>[3x]GGARSDKLLYQAKLA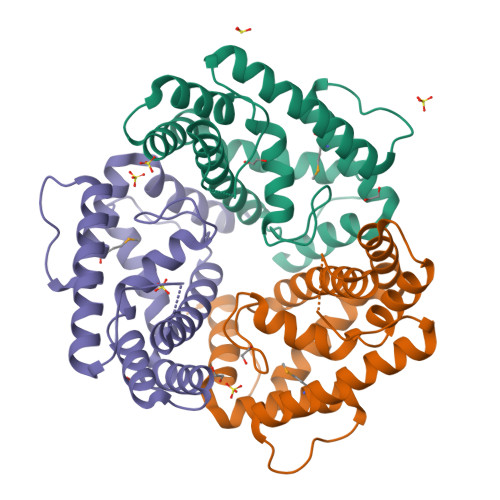LDEDLRLKVVRKMFELRFGEPAPARRSVEQLRGIEGSRVRATYALLAKQYGVTWNGRRYDPKDWEKGDTINQCISAATSCLYGVTEAAILAAGYAPAIGFVHTGKPLSFVYDIADIIKFDTVVPKAFEIARRNPGEPDREVRLACRDIFRSSKTLAKLIPLIEDVLAAGEIQPPAPPEDAQPVAI> DMTQTPSSKSVPVGDTVTINCQA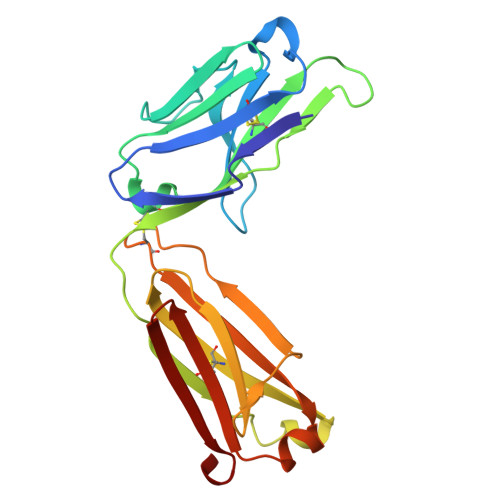SESVYSNNRLSWFQQKPGQPPKLLIYLVSTLASGVPSRFKGSGSGTQFTLTISDVVCDDAATYYCVGYKSSTTDGLAFGGGTEVVVKGDPVAPTVLIFPPAADQVATGTVTIVCVANKYFPDVTVTWEVDGTTQTTGIENSKTPQNSADCTYNLSSTLTLTSTQYNSHKEYTCKVTQGTTSVVQSFNRGDC>HEAGEFFMRAGSATVRPTEGAGGTLGSLGGFSVTNNTQLGLTFTYMATDNIGVELLAATPFRHKIGTRATGDIATVHHLPPTLMAQWYFGDASSKFRPYVGAGINYTT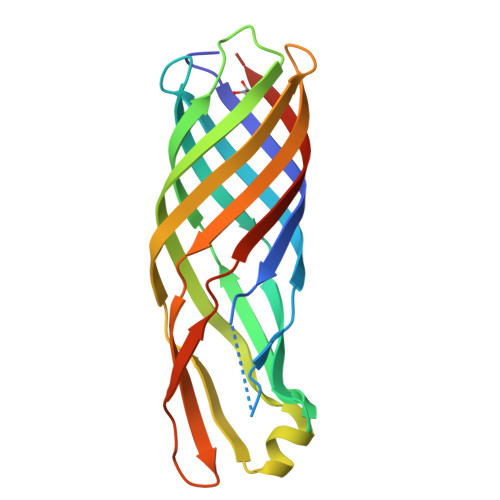FFDNGFNDHGKEAGLSDLSLKDSWGAAGQVGVDYLINRDWLVNMSVWYMDIDTTANYKLGGAQQHDSVRLDPWVFMFSAGYRFHHHHHH[6x]I-PpoI is a well-characterized intron-encoded homing endonuclease member of the physarum polycephalum slimemold. A large subfamily of one-metal-ion-dependent nucleases consist of histidine-metal (His-Me) nucleases that perform critical tasks in biological pathways such as apoptosis, extracellular defense, intracellular immunity (CRISPR–Cas9), and intron homing (homing endonuclease). Surrounded by two beta sheets and an alpha helix, the His-Me nucleases active sites all contain a single metal ion, a histidine, and an asparagine. The asparagine residue helps to stabilize metal ion binding whereas the strictly conserved histidine is suggested to deprotonate a nearby water for nucleophilic attack toward the scissile phosphate.

To confirm if a monovalent metal ion binds in the pre-reaction state, we soaked the I-PpoI crystals in buffer containing Tl+ and detected anomalous electron density at the metal ion-binding site without product formation. (B) Tl+ anomalous signal was detected at the I-PpoI metal ion-binding site after 1800s soaking in 70 mM Tl+. The anomalous map for Tl+ was determined with X-ray at a wavelength of 0.9765 Å and contoured at 3.0 σ. In addition, only one Tl+ was detected by its anomalous signal in the pre-reaction state. Our results support that the monovalent metal ion can bind within the active site without initiating reaction, in corroboration with our biochemical assays. The biochemical and structural results indicate that additional monovalent metal ion may not be necessary for DNA hydrolysis. However, crystal deterioration limited us from soaking the I-PpoI crystals in high concentration of Tl+ for in crystallo reaction.

>[2x]ALTNAQILAVIDSWEETVGQFPVITHHVPLGGGLQGTLHCYEIPLAAPYGVGFAKNGPTRWQYKRTINQVVHRWGSHTVPFLLEPDNINGKTCTASHLCHNTRCHNPLHLCWESLDDNKGRNWCPGPNGGCVHAVVCLRQGPLYGPGATVAGPQQRGSHFVV5-chloranyl-3-phenyl-1~{H}-indole-2-carboxamide 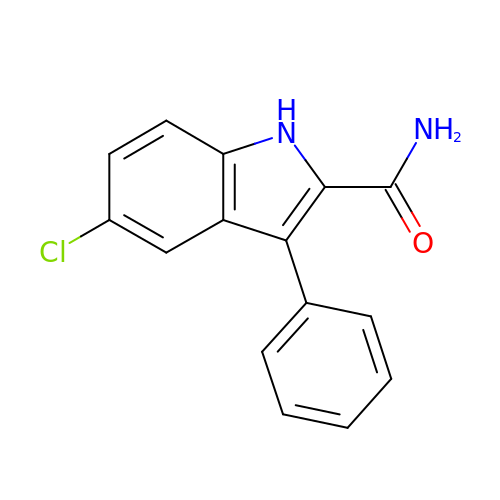| C15 H11 Cl N2 O | ASGAHGHLFFGPBN-UHFFFAOYSA-N>MSISISYSTTYSGWTV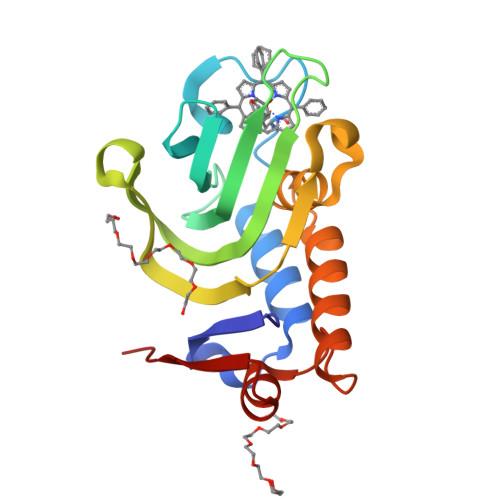ADYLADWSAYFGDVNHRPGQVVDGSNTGGFNPGPFDGSQYALKSTASDAAFIAGGDLHYTLFSNPSHTLWGKLDSIALGDTLTGGASSGGYALDSQEVSFSNLGLDSPIAQGRDGTVHKVVYGLMSGDSSALQGQIDALLKAVDPSLSINSTFDQLAAAGVAHATPAA[4x]>MTATDNARQVTIIGAGLAGTLVARLLARNGWQVNLFERRPDPRIETGARGRSINLALAERGAHALRLAGLEREVLAEAVMMRGRMVHVPGTPPNLQPYGRDDSEVIWSINRDRLNRILLDGAEAAGASIHFNLGLDSVDFARQRLTLSNVSGERLEKRFHLLIGADGCNSAVRQAMASVVDLGEHLETQPHGYKELQITPEASAQFNLEPNALHIWPHGDYMCIALPNLDRSFTVTLFLHHQSPAAQPASPSFAQ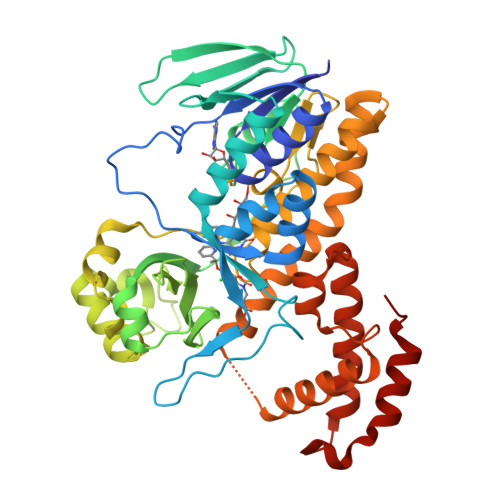LVDGHAARRFFQRQFPDLSPMLDSLEQDFEHHPTGKLATLRLTTWHVGGQAVLLGDAAHPMVPFHGQGMNCALEDAVALAEHLQSAADNASALAAFTAQRQPDALAIQAMALENYVEMSSKVASPTYLLERELGQIMAQRQPTRFIPRYSMVTFSRLPYAQAMARGQIQEQLLKFAVANHSDLTSINLDAVEHEVTRCLPPLSHLS[2x]>VNQSETEIEILAEKIARWARARSAEIERDRRLPDELVTRLREAGLLRATMPREVAAPELAPGRALRCAEAVARGDASAGWCVSIAITSALLVAYLPARSREEMFGGGRGVAAGVWAPRGTARSVDGGVVVSGRWPFCSGINHADIMFAGCFVDDRQVPSVVALNKDELQVLDTWHTLGLRGTGSHDCVADDVFVPADRVFSVFDGPIVDRPLYRFPVFGFFALSIGAAALGNARAAIDDLVELAGGKKGLGSTRTLAERSATQAAAATAESALGAARALFYEVIEAAWQVSHDAEAVPVTMRNRLRLAATHAVRTSADVVRSMYDLAGGTAIYDNAPLQRRFRDAFTATAHFQVNEASRELPGRVLLDQPADVSML[4x]

Our subsequent investigation of one gene cluster (Rv3093c-Rv3095) associated with ethionamide resistance that contained a putative monooxygenase/repressor pair with some resemblance to ethA/ethR, indicates that Rv3094c is likely a flavin-dependent monooxygenase that sulfoxygenates ethionamide, and Rv3095 is its transcriptional regulator. Ethionamide is a second-line anti-tubercular drug used to treat patients infected with multi-drug-resistant or extensively drug-resistant isolates, and is a pro-drug that requires metabolic activation before it can exert its cytotoxic effects. To investigate the mechanism of ethionamide sulfoxygenation by Rv3094c, we solved protein crystal structures of apo-Rv3094c, and Rv3094c in complex with FMN (Rv3094c-FMN) and ethionamide (Rv3094c-FMN-ETH), at resolutions of 1.91 Å, 2.00 Å, and 1.64 Å, respectively. All three crystals contained one tetramer per asymmetric unit, tetramers being formed by two homodimers, the C-terminal domain primarily mediating interactions between the two monomers.

F136 is the main residue involved in FMN binding pocket formation, and its side chain swings out to create the FMN binding pocket. The FMN flavin ring of FAD is held in position by a network of hydrogen bonds (involving G113, W115, and S138) and hydrophobic interactions (involving W80, V114, F136, W174, L179, S184, T347, H351, and F352). (i) A conformational change occurs in F136 and Rv3094c binds reduced FMN. (ii) An electron from reduced FMN then transfers to oxygen, forming a hydroperoxyflavin intermediate. During this process, H351 acts as a proton donor, stabilizing the hydroperoxyflavin intermediate. As Rv3094c is co-transcribed with Rv3093c, a predicted FAD/FMN reductase, and FAD in ACAD family proteins is often reduced by an associated flavoprotein, we reasoned that Rv3093c and Rv3094c may form a two-component system in which Rv3094c is the monooxygenase partner responsible for the sulfoxygenation of ethionamide.> SMLYKELGRTGEEI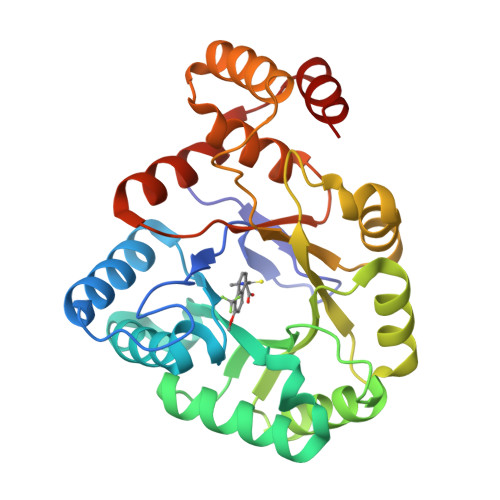PALGLGTWGIGGFETPDYSRDEEMVELLKTAIKMGYTHIDTAEYYGGGHTEELIGKAIKDFRREDLFIVSKVWPTHLRRDDLLRSLENTLKRLDTDYVDLYLIHWPNPEIPLEETLSAMAEGVRQGLIRYIGVSNFDRRLLEEAISKSQEPIVCDQVKYNIEDRDPERDGLLEFCQKNGVTLVAYSPLRRTLLSEKTKRTLEEIAKNHGATIYQIMLAWLLAKPNVVAIPKAGRVEHLRENLKATEIKLSEEEMKLLDSLG>[2x]IPCGKFAMYPAWQPDADFQRQAALWGVALREPVTAEELAAFIAYWQAEGKVFHH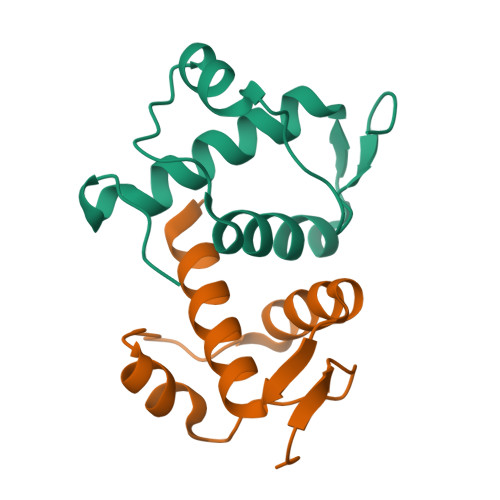IQWQQKLARSVQISRSSNGGMPQRDINSVSEPDNHIPPGFRGHHHHHH Beta-N-acetylgalactosaminidases (β-NGAs) hydrolyze the different β-GalNAc linkages of various glycans to modulate the length, combination, and abundance of glycans. Despite low sequence similarity, the crystal structures of these enzymes demonstrate that all enzymes share a prototype structure and have diversified their substrate specificities (oligosaccharide-releasing, oligosaccharide/monosaccharide-releasing, and monosaccharide-releasing) through the accumulation of mutations and insertional amino acid sequences. The overall structure of these enzymes is similar to that of CpNga123 and BvGH123, which consist of a β-sandwich domain at the N-terminus and a (β/α)8-barrel domain encompassing the catalytic region. Among Groups 1–4 and GH123, the DE motif is located at the same position, suggesting that these enzymes adopt the substrate-assisted catalysis reported for GH123 MR-β-NGAs.

Surprisingly, Group 1 NgaCa displayed strictly OR-type enzymatic activity and acted solely on Galβ1-3GalNAc-β-pNP. NgaCa in Group 1 had the simplest structure among the enzymes analyzed. The active site of NgaCa possesses a cleft shape that allows oligosaccharides to pass through to the −2 subsite, enabling oligosaccharide binding and OR-type β-NGA activity. Furthermore, three characteristic tryptophan residues (W197, W218, and W249) are located in the subsites −2 and −3. A docking model of NgaCa with oligosaccharide suggested that these tryptophan residues may play a role in a stacking-type interaction with sugars located in subsites −2 and −3. This structural feature indicated that Group 1 enzymes may act on the inner regions of longer sugar chains, in addition to disaccharides from the non-reducing end (e.g., Galβ1-3GalNAc-β-pNP). By contrast, no inhibition was observed in Group 1 OR-β-NGA even at a concentration of 100 μM (green). This difference in the inhibitory activity of Group 1 enzymes can be explained as follows: the monosaccharide reaction intermediate-mimicking inhibitor (GalNAc-thiazoline) does not bind tightly to the substrate pocket of OR-type enzymes. The increased number of residues could potentially reinforce substrate recognition in Group 4 and GH123 enzymes. Additional structural analyses (comparison of crystal structure with AlphaFold2 predicted structure of NgaCa, comparison of apo1-form and apo2-form of NgaCa, and comparison of GalNAc-thiazoline-bond form and GlcNAc-thiazoline-/apo-form of NgaAt, NgaDssm, and NgaP2) data are illustrated in Supplementary Fig. 13.

> GPGMANTQKTLSLSVWTASSQERVRQDDPAGESLNIELFAARGEYESFQVALKAPEGEHRNVHFVVSDLKGTGDSFISKSNLTLYREHYVYISESSPQRGTVLPEGPGWYPDALIPFIDPATNEPPSGGELIAVPFALENNSNQVIWVDIQVPRDAEAGHYSGSYIVSSEHGEVTGQISLTVWNFELPLKPSLKSTFLIWSSRKKSTVEELLKHKLMCQQWNLSEEEKGAAPTSEGEWIEKYGVNCSGLGFWSKADTFNGVMPPPPTVEEIQAAASAHPSNLFLYNYTADEIGHYTSLYEPIKAWARNLHEAGVANLITMAPVPELYDDGSGSGRSAVDIWVILPLQYDKDRIQEVLAKGDEVWSYNCCVQDDYSPKWQIDFNPIEYRIQPGFINQSLGMTGILYWRVDFWTEDPWHDVLTLRADGMEFNGEGMLVYPGEQVGIDGVVPSIRLKAIRKGIEDYEYIEILKNLGHEQWALEISQSVGPDWHNWTKDHHKLEWARKQLGERINDLMTK>MASNRRYQEPQNRDISSRSNGKNPFKRSTGRKVSNVIIIILCVVFSGLGGVIVYAHGLLAGMYQNLDSTVLDSSAKESLTASSNSSNTSSIAEIPANIDGTLIKDPMVLNIMLFGSDERPGETGYGRSDTMMLLSIDNRNKKLKLTSFMRDTYVNVPEWGDTKLTHAYSYGGPALAIETIERNFGIDIDRYAVVYFDTFPGIVDTLGGIEVEMTQTEADVMNESVGPEFANFTEGKNTLNGATALVYVRIRYGVGDDFGRTQRQRDFMLQVLNKVKGTRDV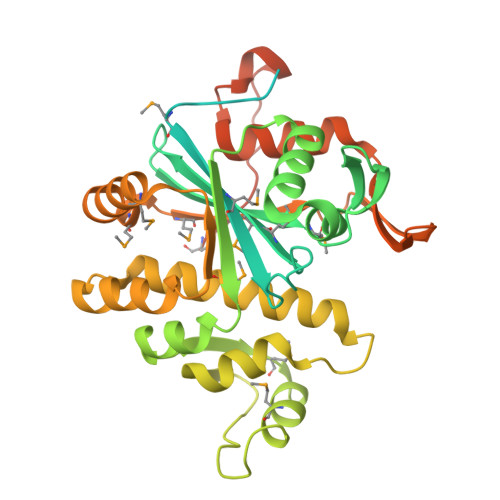GTLLTLLTKILPGVTTNISVNEMAGLAGGAISSYMDYPMYQFRLPEDGAFSAVDVDAGNVLAIDDWDAAREHLQRFIYEDTVDPIYGPSTETYGSEMGSSKTAGSSSLSGYSEDLEHHHHHH[2x]> RSPRLVGGDIPCSGRVEVQHGDTWGTVCDSDFSLEAASVLCRELQCGTVVSLLGGAHFGEGSGQIWAEEFQCEGHESHLSLCP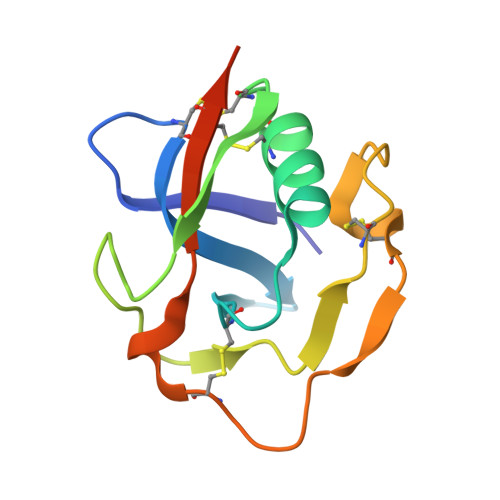VAPRPDGTCSHSRDVGVVCSTRTGHHHHHH> MGDLSCPEGLEELLSAPPPDLGAQRRHGWNPKDCSENIEVKEGGLYFERRPVAQSTDGARGKRGYSRGLHAWEISWPLEQRGTHAVVGVATALAPLQTDHYAALLGSNSESWGWDIGRGKLYHQSKGPGAPQYPAGTQGEQLEVPERLLVVLDMEEGTLGYAIGGTYLGPAFRGLKGRTLYPAVSAVWGQCQVRIRYLGERGSHHHHHH;> KDIN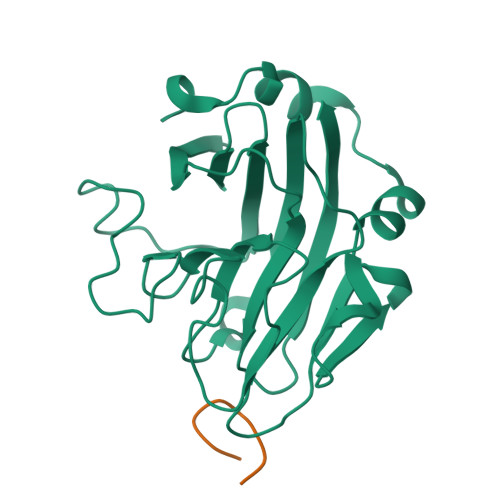NNVEK>SMEPRVEVMDPAGGPRGVLPRPCRVLVLLNPRGGKGKALQLFRSHVQPLLAEAEISFTLMLTERRNHARELVRSEELGRWDALVVMSGDGLMHEVVNGLMERPDWETAIQKPLCSLPAGSGNALAASLNHYAGYEQVTNEDLLTNCTLLLCRRLLSPMNLLSLHTASGLRLFSVLSLAWGFIADVDLESEKYRRLGEMRFTLGTFLRLAALRTYRGRLAYLPVGRVGSKTPASPVVVQQGPVDAHLVPLEEPVPSHWTVVPDEDFVLVLALLHSHLGSEMFAAPMGRCAAGVMHLFYVRAGVSRAMLLRLFLAMEKGRHMEYECPYLVYVPVVAFRLEPKD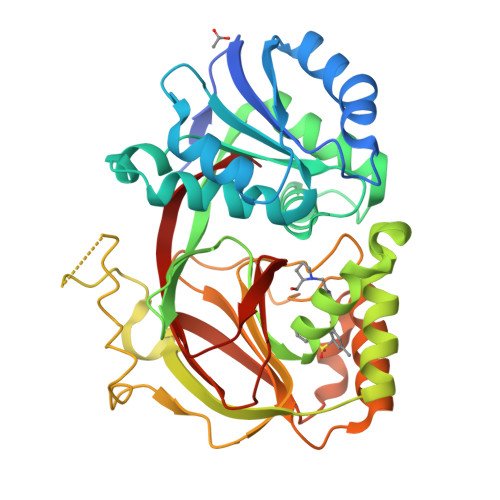GKGVFAVDGELMVSEAVQGQVHPNYFWMVS[2x]>[2x]GSSHHHHHHSSGLVPRGSMSTSWSDRLQNAADMPANMDKHALKKYRREAYHRVFVNRSLAMEKIKCFGFNMDYTLAVYKSPEYESLGFELTVERLVSIGYPQELLSFAYDSTFPTRGLVFDTLYGNLLKVDAYGNLLVCAHGFNFIRGPETREQYPNKFIQRDDTERFYILNTLFNLPETYLLACLVDFFTNCPRYTSCETGFKDGDLFMSYRSMFQDVRDAVDWVHYKGSLKEKTVENLEKYVVKDGKLPLLLSRMKEVGKVFLATNSDYKYTDKIMTYLFDFPHGPKPGSSHRPWQSYFDLILVDARKPLFFGEGTVLRQ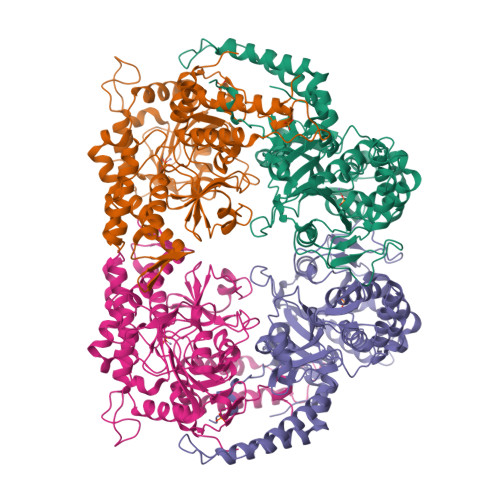VDTKTGKLKIGTYTGPLQHGIVYSGGSSDTICDLLGAKGKDILYIGDHIFGDILKSKKRQGWQTFLVIPELAQELHVWTDKSSLFEELQSLDIFLAELYKHLDSSSNERPDISSIQRRIKKVTHDMDMCYGMMGSLFRSGSRQTLFASQVMRYADLYAASFINLLYYPFSYLFRAAHVLMPHESTVEHTHVDINEMESPLATRNRTSVDFKDTDYKRHQLTRSISEIKPPNL5-{(3R)-3-methyl-4-[(1R,2R)-2-methylcyclopropane-1-carbonyl]piperazin-1-yl}-3-(1-methyl-1H-pyrazol-4-yl)pyrazine-2-carbonitrile | C19 H23 N7 O | 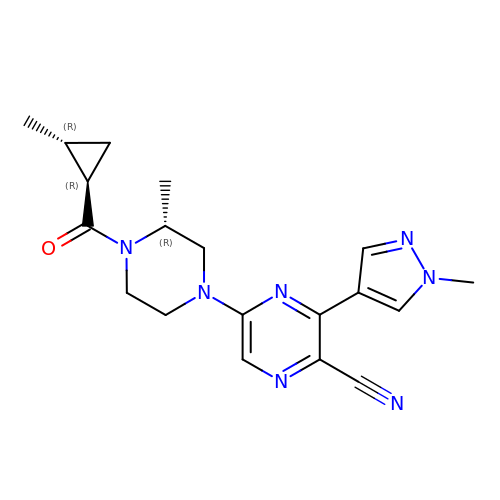GXEXIUKEWXZCEF-UMVBOHGHSA-N>GSSGSSGMASSCAVQVKLELGHRAQVRKKPTVEGFTHDWMVFVRGPEHSNIQHFVEKVVFHL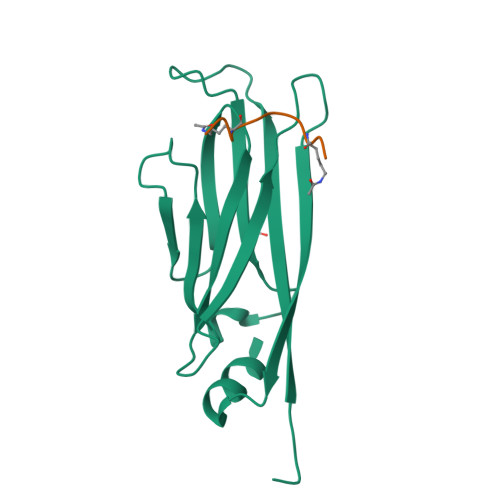HESFPRPKRVCKDPPYKVEESGYAGFILPIEVYFKNKEEPRKVRFDYDLFLHLEGHPPVNHLRCEKLTFNNPTEDFRRKLLKA[2x];>KGGKGLGKGG[2x]> ADQKLQDAKTDAKQQITNFTGLTEPQKQALENIINQQTSRANVAKQLSHAKFLNGKMEELKVAVAKASLVRQNSNYINEDVSEKE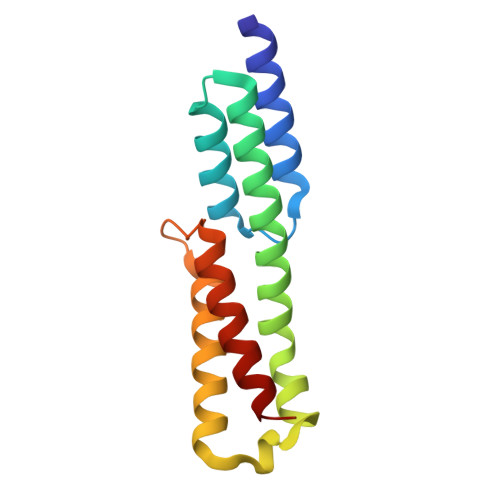AYEQAIAKGQEIINSENNPTISSTDINRTIQEINDAEQNLH>[3x]MV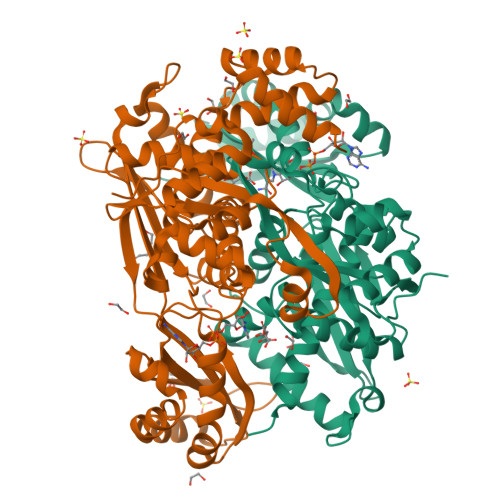ADSRLPNFRALTPAQRRDFLADACGLSDAERALLAAPGALPLALADGMIENVFGSFELPLGVAGNFRVNGRDVLVPMAVEEPSVVAAASYMAKLAREDGGFQTSSTLPLMRAQVQVLGVTDPHGARLAVLQARAQIIERANSRDKVLIGLGGGCKDIEVHVFPDTPRGPMLVVHLIVDVRDAMGANTVNTMAESVAPLVEKITGGSVRLRILSNLADLRLARARVRLTPQTLATQDRSGEEIIEGVLDAYTFAAIDPYRAATHNKGIMNGIDPVIVATGNDWRAVEAGAHAYASRSGSYTSLTRWEKDAGGALVGSIELPMPVGLVGGATKTHPLARLALKIMDLQSAQQLGEIAAAVGLAQNLGALRALATEGIQRGHMALHARNIALVAGATGDEVDAVARQLAAEHDVRTDRALEVLAALRARA> MKKWIYVVLVLSIAGIGGFSVHAASSAHEKHLNVSKMNVDDEFKDTDGTFILHDLQKDQTFVYNRKRANQRQTPQSTFKVVNALIGLQVKAVRDEYDVKRWDGVKREFESWNRDHTLGSAMRESAIWYYQALARDIGEERMKTWLHTLSYGNEDISGGIDQFWLQSSLTISPLEQETFLEKLAKEELPFDKPVMKIVKRMMIQEEGDHYTLYGKTGTRLTDMGLGWFVGFIKTEHGSYV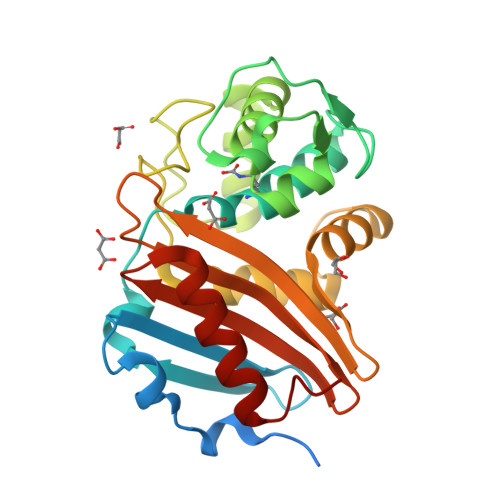FVTNVDDSGTKAKNITVDILKKYGLITS>MKTFAAYVIIACLSSTALAGSITENTSWNKEFSAEAVNGVFVLCKSSSKSCATNDLARASKEYLPASTFKIPNAIIGLETGV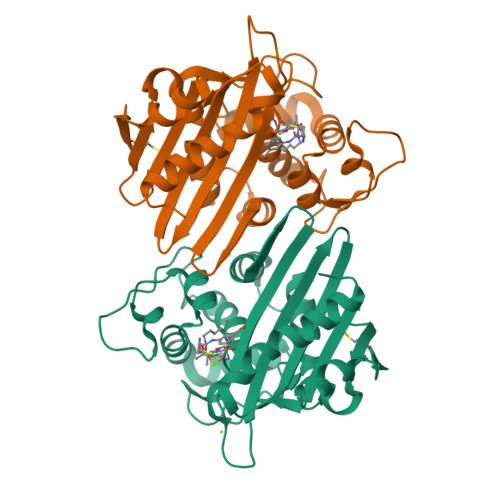IKNEHQVFKWDGKPRAMKQWERDLTLRGAIQVSAVPVFQQIAREVGEVRMQKYLKKFSYGNQNISGGIDKFWLEGQLRISAVNQVEFLESLYLNKLSASKENQLIVKEALVTEAAPEYLVHSKTGFSGVGTESNPGVAWWVGWVEKETEVYFFAFNMDIDNESKLPLRKSIPTKIMESEGIIGG[2x]> MSQ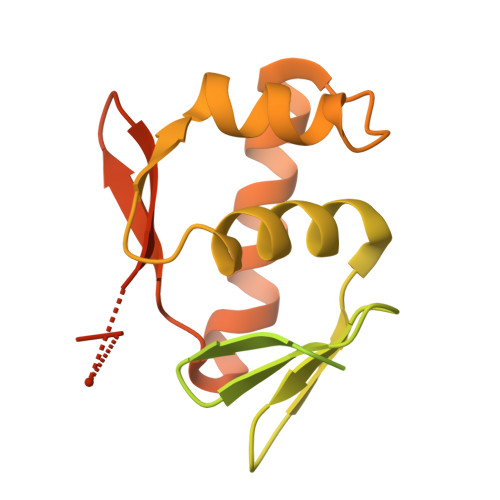EQGKIYIVEDDMTIVSLLKDHLSASYHVSSVSNFRDVKQEIIAFQPDLILMDITLPYFNGFYWTAELRKFLTIPIIFISSSNDEMDMVMALNMGGDDFISKPFSLAVLDAKLTAILRRSQQFIQQELTFGGFTLTREGLLSSQDKEVILSPTENKILSILLMHPKQVVSKESLLEKLWENDSFIDQNTLNVNMTRLRKKIVPIGFDYIHTVRGVGYLLQNDPSSSVDKLAAALEHHHHHH> 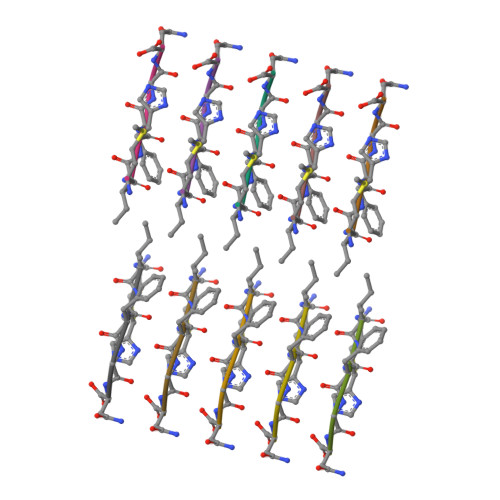MIHFGN> MSQAGDTLNDVIQDPTRRNKLINDNNLLKGIIMGRDGPVPSSRELIVRPDTLRAIINNRATIETTTMEAEFTETLMESNYNSASVKVSAPCITANSEYSESSSFKNTETEKSM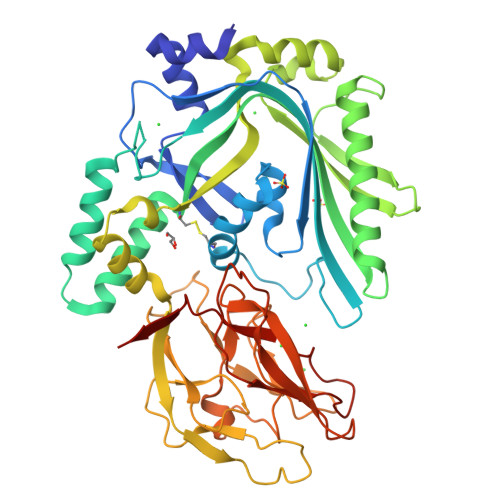YTSSRYLFPQGRIDFTTPDSGFDDVIKLSPQFTSGVQAALAKATGTEKREALQNLFQEYGCVFRTKVHIGGVLSAHTMETFSRSENETEVKQDVKAGLEGAVKGWGGGATAGHGNTQGTITTSQNRKLNVKYIVNGGDYTKIQNTEEWVASTNQSEHWRVIEVTEVTAVADLLPQPIRGQVKDLLKPLLGKWVDVEKVPGLESLPVSVYRPKGAIPAGWFWLGDTADASKALLVKPTLPARSGRNPALTSLHQGSGMTEQPFVDLPQYQYLSTYFGSFAHDTPPGSTLRGLRPDHVLPGRYEMHGDTISTAVYVTRPVDVPFPEDEAFDLKSLVRVKLPGSGNPPKPRSALKKSMVLFDSGEK(methoxymethyl)cyclopropane | C5 H10 O | 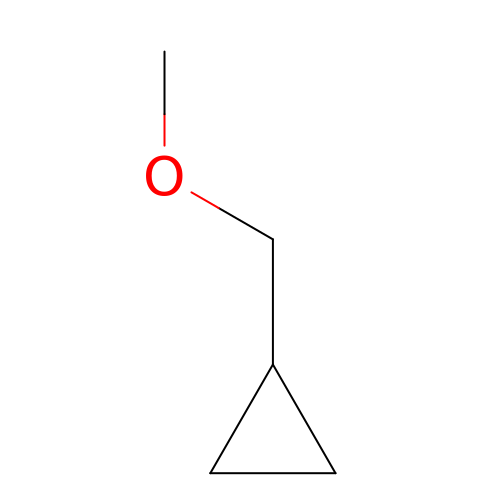XZUHEKNCBBQEBT-UHFFFAOYSA-N>[2x]DDLYRQSLEIISRYLREQATGSKDSKPLGEAGAAGRRALETLRRVGDGV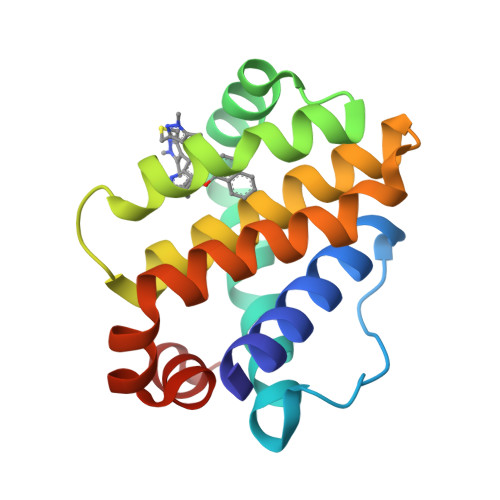QRNHETAFQGMLRKLDIKNEDDVKSLSRVMIHVFSDGVTNWGRIVTLISFGAFVAKHLKTINQESCIEPLAESITDVLVRTKRDWLVKQRGWDGFVEFFHV> GTGRPEWIWLALGTALMGLGTLYFLVKGMGVSDPDAKKFYAITTLVPAIAFTMYLSMLLGYGLTMVPFGGEQNPIYWARYADWLFTTPLLLLDLALLVDADQGTILALVGADGIMIGTGLVGALTKVYSYRFVWWAISTAAMLYILYVLFFGFTSKAESMRPEVASTFKVLRNVTVVLWSAYPVVWLIGSEGAGIVPLNIETLLFMVLDVSAKVGFGLILLRSRAIFGEAE

The primary function of bR is that of a light-driven proton pump, where trans to cis isomerization of a covalently bound retinal chromophore starts a series of conformational changes necessary for directional transport against a concentration gradient. Structurally, bR shares the seven trans-membrane α-helical topologies typical for other rhodopsins, as well as G protein-coupled receptors. The primary reaction from the bR dark state to the K-intermediate is the isomerization of retinal from the all-trans conformation to a twisted 13-cis conformation that stores a significant part of the initial photoenergy. Here, we investigate the effects of increasing laser power density on the light-driven proton pump bacteriorhodopsin with a focus on the K-intermediate that accumulates just after the excited retinal chromophore returns to the electronic ground state.

The thermal load can be followed over time when analyzing the atomic B-factor difference between light and dark datasets collected at 10 ps, 100 ps, 1 ns, and 10 ns delays excited at 1281 GW/cm2. The relative B-factor difference on the counterion cluster and retinal continually decays before disappearing after 10 ns where the heat is nearly evenly distributed throughout the crystal as evident from the maximally expanded unit cell.> MKDGKQEKVLTTCPYCGTGCGLYLKVENEKIVGVEPDKLHPVNQGELCIKGYYGYKYVHDPRRLTSPLIKKNGKFVPVSWDEALNFIANGLKKIKSEYGSDAFAMFCSARATNEDNYAAQKFARAVIGINNVDHCARLCHAPTVAGLAMTLGSGAMTNSIPEISTYSDVIFIIGSNTAECHPLIAAHVIKAKERGAKLIVADPRMNAMVHKADIWLRVPSGYNIPLINGMIHIIIKEGLVKTDFVKNHAVGFEEMAKAVEKYTPEYVEELTGIPKKDLIKAARFYGQAQAAAILYSMGVTQFSHGTGNVVSLANLAVITGNLGRPGAGICPLRGQNNVQGACDVGALPNVLPGYLDVTKEQNRERFEKVWGVKLPSNIGLRVTEVPDAILNKRVRALYIFGENPIMSDPDSDHLRHALEHLDLLIVQDI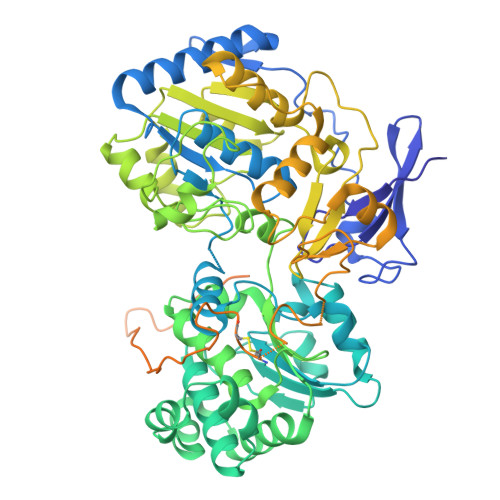FLTETARLAHVVLPAACWAEKDGTFTNTERRVQRVRKAVEAPGEAKPDWWIFSQIAERMGYTGMQYNNVQEIWDEVRKIVPEKFGGISYARLEKEKGLAWPCPTEDHTGTPILYLGGKFATPSGKAQMYPVIFYPNTCICDEGAEKQDFNHVIVGSIAELPDEEYPFTLTTGRRVYHYHTATMTRKSPVIDQIAPQELVEINPQDATRLGINDGDFLRVSTRRGYVATRAWVTERVPKGTIFMTFHYWEACCNELTNTASDAICCIPEFKVAAAKVEKISQVEAQAILKEKIEKYQVELEKDVANMLAKEKGGK> MRGQGRKESLSDSRDLDGSYDQLTGHPPGPTKKALKQRFLKLLPCCGPQALPSVSENSVDDEFELSTVCHRPEGLEQLQEQTKFTRKELQVLYRGFKNECPSGIVNEENFKQIYSQFFPQGDSSTYATFLFNAFDTNHDGSVSFEDFVAGLSVILRGTVDDRLNWAFNLYDLNKDGCITKEEMLDIMKSIYDMMGKYTYPALREEAPREHVESFFQKMDRNK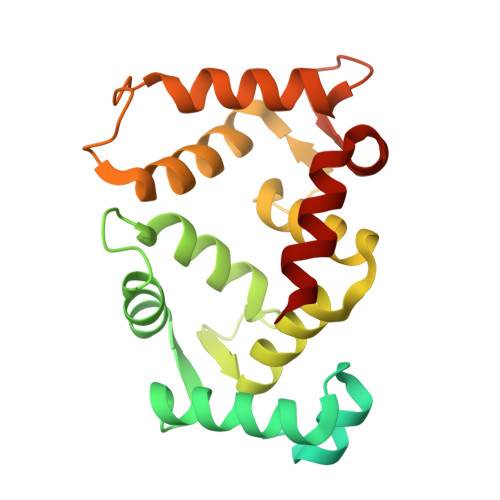DGVVTIEEFIESCQKDENIMRSMQLFDNVI> KAQDDSTPDSLFAGLVGEYYGTNSQLNNISDFRALVDSKEADATFEAANISYGRGSSDVAKGTHLQEFLGSDASTLSTDPGDNTDGGIYLQGYVYLEAGTYNFKVTADDGYE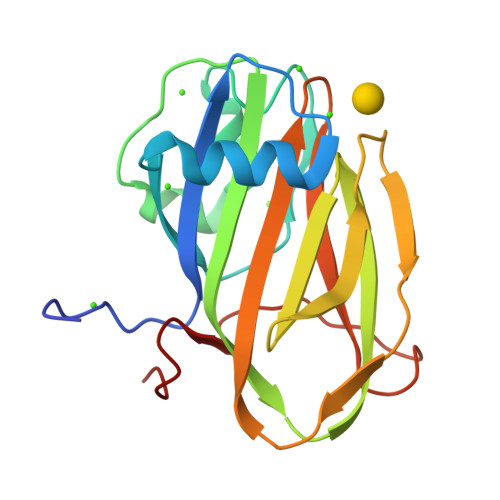ITINGNPVATVDNNQSVYTVTHASFTISESGYQAIDMIWWDQGGDYVFQPTLSADGGSTYFVLDSAILSSTGETPY>[16x]GAMAEEYSWDSYLNDRLLATNQVSGAGLASEEDGVVYACVAQGEESDPNFDKWSLFYKEDYDIEVKTTKTINEGQTILVVFNEGYAPDGVWLGGTKYQFINIERDLEFEGYN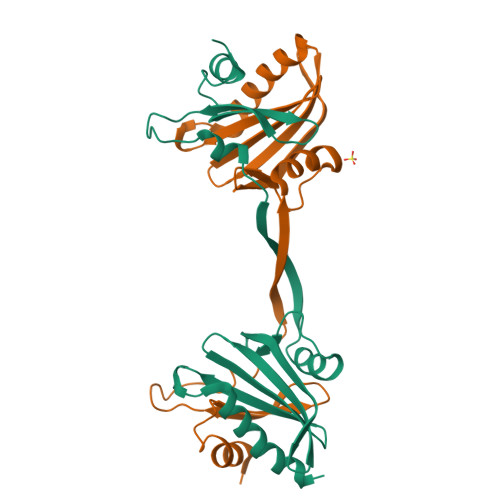FDVATCAKLKGGLHLVKVPGGNILVVLYDEEKEQDRGNSKIAALTFAKELAESSQLQ> SAKAAEGYEQIEVDVVAVWKEGYVYENRGSTSVDQKITITKGMKNVNSETRTVTATHSIGSTISTGDAFEIGSVEVSYSHSHEESQVSMTETEVYESKVIEHTITIPPTSKFTRWQLNADVGGADIEYMYLIDEVTPIGGTQSIPQVITSRAKIIVGRQIILGKTEIRIKHAERKEYMTVVSRKSWPAATLGHSKLFKFVLYEDWGGFRIKTLNTMYSGYEYAYSSDQGGIYFDQGTDNPKQRWAINKSLPLRHGDVVTFMNKYFTRSGLCYDDGPATNVYCLDKREDKWILEVVGLVPRGSGHHHHHH

Lysenin from the earthworm Eisenia fetida is a pore-forming protein that specifically interacts with sphingomyelin (SM) and may confer innate immunity against parasites by attacking their membranes (Bruhn et al., 2006; Cooper et al., 2001). The structure reveals that lysenin has two domains. The topology of the lysenin structural fold establishes it as a member of the aerolysin family of pore-forming proteins (Szczesny et al., 2011), which appears thus to be conserved from bacteria to annelids. Here we report the crystal structure of lysenin alone, and in complex with the sphingomyelin headgroup phosphocholine (POC), and with SM itself.

The crystal structure of lysenin was first determined in space group P6522, with one molecule per asymmetric unit (a.u.), by multiple isomorphous replacement with anomalous scattering (MIRAS, one SeMet and one Hg derivative) and then in space group P1 with four molecules per a.u. by molecular replacement. In the crystal form with space group P6522 the protein was found in complex with a phosphocholine molecule (lysenin:POC). This lipid headgroup binds specifically within the β-trefoil via a hydrogen bond network involving residues Tyr233, Ser227, Tyr282, and a salt bridge interaction with Lys185. Residue Gln229 is the gate regulating access to the POC binding pocket: in the apo forms of lysenin, Gln229 is in a closed conformation, blocking the entrance to the POC binding site, but has opened in the POC bound state. Lys185 aids in defining the gate, as it is in a different conformer in the apo form, preventing interaction with the phosphate moiety. Unlike other β sheeted POC-binding proteins, such as staphylococcal LukF, the POC pocket of lysenin does not involve cation-π interactions between the electron-rich systems of the tyrosine aromatic rings (Olson et al., 1999), but it is similar to that found in actinoporins (Mancheño et al., 2003). We also find an additional POC-binding site, which indicates how lysenin might be guided in its attack on the target membrane. We suggest that lysenin interacts with the membrane initially by binding of POC in lipids such as SM through its β-trefoil, after attraction to the membrane surface through charge-charge affinity; it will then bind the full length of SM. The structures described in this study suggest that lysenin interacts with POC—not necessarily only that of SM but also from phosphocholine lipids—via its lectin domain prior to pre-pore assembly and pore formation.Agmatinase (AGM) is the enzyme that catalyzes the hydrolysis of agmatine in urea and putrescine, and to date, E. coli AGM (EcAGM) is the best agmatinase kinetically characterized. AGMs belong to the ureohydrolases enzymes family, containing all the conserved residues of this family similar to arginases (ARG), proclavaminic acid amidino hydrolases (PAH), guanidinopropionase (GpuA), and guanidinobutyrase (GbuA). The hexamer as oligomeric state tallies as is described to other bacterial agmatinases and arginases from bacteria and plants.

Two structures in different space groups were solved by X-ray crystallography, one at low resolution (3.2 Å), including a guanidine group; and other at high resolution (1.8 Å) which presents urea and agmatine in the active site. For 1.8 Å resolution structure, the asymmetric unit of the crystal contains one chain of protein, an urea molecule, and agmatine in the channel formed by the loops A and B, and three manganese atoms; two at the active site, and one at the interfaces with the other two asymmetric units. However, this agmatine is in a non-catalytic position, away from the site of the Mn2+ ions, where an urea molecule is present. The presence of this agmatine probably comes from the expression and its location does not allow visualize a clear role in catalysis, possibly being an artifact of crystallization. Mn2+-bridging water (w1) is possible to identify between Mn2+ ions in the high-resolution structure, which has been described as an essential nucleophile for ureohydrolases catalysis. Two types of intra-trimer interactions can be observed, one formed by the association between two adjacent monomers (monomer-monomer interaction, i.e., A-B) and the other where one Mn2+ ion and TRIS molecule are found, implicating the interactions of the three monomers (trimeric interactions). H-bonds mediate a similar intermonomer association between the backbone from Pro240 and Ala237 and the OH- of a TRIS buffer molecule. The solved structures in complex with guanidine and urea provide insights into the catalytic mechanism of the EcAGM. The primary interaction of guanidine occurs with, His126, Asp153, His163, Asp230, Asp232 and Glu274, whereas urea can interact directly only with Asp153, Asp230, and Glu274. The structures with guanidine and urea made it possible to propose EcAGM’s catalytic mechanism and provide evidence of the importance of His163 as a proton shuttle and a stabilizer of the transition state in bacterial ureohydrolase.

> MSTLGHQYDNSLVSNAFGFLRLPMNFQPYDSDADWVITGVPFDMATSGRAGGRHGPAAIRQVSTNLAWEHNRFPWNFDMRERLNVVDCGDLVYAFGDAREMSEKLQAHAEKLLAAGKRMLSFGGDHFVTLPLLRAHAKHFGKMALVHFDAHTDTYANGCEFDHGTMFYTAPKEGLIDPNHSVQIGIRTEFDKDNGFTVLDACQVNDRSVDDVIAQVKQIVGDMPVYLTFDIDCLDPAFAPGTGTPVIGGLTSDRAIKLVRGLKDLNIVGMDVVEVAPAYDQSEITALAAATLALEMLYIQAAKKGE>MITRETLKSLPANVQAPPYDIDGIKPGIVHFGVGNFFRAHEAFYVEQILEHAPDWAIVGVGLTGSDRSKKKAEEFKAQDCLYSLTETAPSGKSTVRVMGALRDYLLAPADPEAVLKHLVDPAIRIVSMTITEGGYNINETTGAFDLENAAVKADLKNPEKPSTVFGYVVEALRRRWDAGGKAFTVMSCDNLRHNGNVARKAFLGYAKARDPELAKWIEENATFPNGMVDRITPTVSAEIAKKLNAASGLDDDLPLVAEDFHQWVLEDQFADGRPPLEKAGVQMVGDVTDWEYVKIRMLNAGHVMLCFPGILVGYENVDDAIEDSELLGNLKNYLNKDVIPTLKAPSGMTLEGYRDSVISRFSNKAMSDQTLRIASDGCSKVQVFWTETVRRAIEDKRDLSRIAFGIASYLEMLRGRDEKGGTYESSEPTYGDAEWKLAKADDFESSLKLPAFDGWRDLDTSELDQKVIVLRKIIREKGVKAAIP[2x]

In this study, we heterologously expressed and fully characterized a recombinant polyol-specific long-chain GoSLDH. Based on the conserved catalytic motif (KXXXXHXXH) in polyol-specific long-chain dehydrogenase, GoSLDH can be grouped into the subfamily of polyol-specific long-chain dehydrogenases. The observed results suggested that GoSLDH is highly specific towards D-sorbitol, mannitol, and D-arabinitol. Measurement of activity with D-sorbitol as a substrate suggested that GoSLDH is exclusively an NADP+-dependent enzyme, resulting in only 2.5% relative activity with NAD+.

The identified GoSLDH had 32–82% sequence identity with polyol-specific long-chain dehydrogenase family enzymes. Further, the catalytic region of Pseudomonas fluorescens MDH (PfMDH) was identified as the previously suggested conserved sequence (KXXXXNXXH) of polyol-specific long-chain dehydrogenase. This GoSLDH alignment (Q9KWR5) revealed the presence of three highly conserved residues, Lys294, Asn299, and His302, that have been found in other known polyol-specific long-chain dehydrogenases. In addition, GoSLDH possessed the active site residues of Asp190, Val228, Lys294, and Asp299. The structure of GoSLDH and PfMDH bound with D-sorbitol lacked sufficient detail to reveal precisely how it bound. To understand the binding conformation of D-sorbitol along with GoSLDH and PfMDH, molecular docking was performed. D-Sorbitol formed strong interactions of five hydrogen bonds with GoSLDH, with Asn190, Lys294, and Leu191 playing the roles of interacting amino acids. In addition to the hydrogen bonding network, the amino acids Met227, Val287, Ile295, and Phe384 showed hydrophobic bonding with the D-sorbitol in GoSLDH. The distance between Lys294 and the O2 hydrogen atom of D-sorbitol was 2.35 Å, which favors close contact. Given the shorter distance between Lys294 and the O2 hydrogen of the substrate, it seems that GoSLDH could abstract a proton more efficiently than PfMDH. Further, the high activity of GoSLDH was analyzed in a structural analysis together with CV and ITC studies. These observations suggested that recombinant GoSLDH is more catalytically efficient than other SLDH or MDH due to the close proximity of D-sorbitol to the catalytic residue, along with high binding affinity.>[6x]MSTLNKHISIPKDMSSKDDLDFHFLREEGIRYIKELGSNFWTDYNTHDPGITMLEVLCYAISDLGNRINIPIEDLIANEEGGVKGQFYKVQEILPSAPTSELDLRKLFIDIEGIKNCWIKRERVTVFADLKNQKLSYEKTIWEDLKENQKAQFDLKGLYRILVETEDADKVLSESLEKAVFTKFHANRNLCEDLIKVEKVATEPISVCANVEVAPEADEELIHAQILIAIEDYLAPSPRHYSLKQMVDKGYTMDEIFEGPFLENGFIDTVELKASELRKEVRLSDIINIIMSIDGVKIVKEITLGNCDENDGIENNQWVICIPENKKPKLCKKTTINYFKGILPINLNPVRVDNHKSKILASRLENDLKAKDDLEPAIPQGTFADWGEYSSIQHEFPETYGISDIGLPPKLGVKRAVLARQLKGYLLFFDQILASYFEHLSKIKSLLSLDQGPSFTYFTQAIKDIKDVEELFKDPTLLENDEELTKSLIGKLDDTIERRNQLMDHLIARFAENFSSYAFLMKFLYGESTDEIVLQDKQSFLREYKEISRERGEGFNFYEQSNDNLWDTLNVSGAQKRISKLVGVKDYSRRNLSDTAVEIYRYEHVDGNWVYRWRIRDENGKVLLSATTSYPTYNSAGNEMYFAILKILETPLSDLEKLLEVNFRNENEAGSFHFHKAATSNKFSFDIINPVIDSESSSDFIVAKQYTYYPDRTQAVLGAISLLNFIKYTFTEEGIYLVEHILLRPSPLDPEYLAMQTDAGKEYIEGNFLPFCSDDYENCKMIDPYSFRVSIVLPGFTYRFANKDFRDYLENLIREELPAHIVAKICWIGYRKGEEPELFQEDVENPETPIFKENQLEIFEKAYKNYLFELTDIHKRKGFIASMNKYNQVLNEMTSSLTGLHTIYPTGRLYDCEDEEEELDGKLILGKTNLGTL;>MSENCNHIVTTLKRDGTGRRDLLDPKLAPESVQLQDFELSDWLIFALNFARKIHFFPSDLANEPLGDWR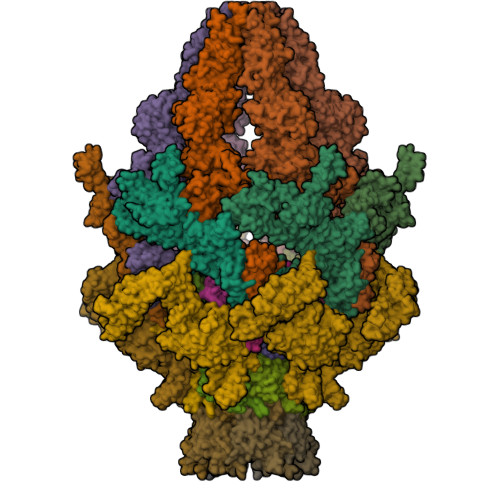NFFSTIVSDKTLISDIENLDDFEKLRGNIEEFLAAYDQSGKLTPHLTLFVSFLKLLETSKKRFNQLTKRHLDFYYQEILHLEKQALSPDHVFLIFELAKNVSQEKLDEGTEVDGGKDDTGKKNTYLTSFETVLNKTKVGQLKSLYNEISVEKEEIKELNTPISTGTFVMAPMANSFDGLGEDFPKGSEKWWPFGYTKICNASTVLPALPKARLGCSISSKLLKLSEGTRDIILEFTFNKPILPNGEDYTALNKAMSIELTGEKGWIAGLPMTLKSDSGINSGSKKMKLSLTLDSEQPAVVPYQTELHEGSYEVDEPLLRVLFKTNEKEGYNLYRLFNENVLTDLKITVEVSDITSVQLENDLGVLNPQKPFFPFGPRPIKGSSFIVKYPEAMEKPVTAISYQMDYLNLPENLVNHYSAYTIGDDEPLVSDMDYFSVKSFPKSSNDSDQLFSEKSGGGYESDFEFQIENGVWESGLKKELKISLERSFLHEKYAHYFTLVAISKDTDPTIELLPNEPYAPLAENLVLGYTAISSIDFSSSSSENQVSLIHEMPFGFQQVFTPGDTDNSLYLVPDYCHGGELYIGLENGKNLQQVTLLLQFLEGSENPDITDIFTGNQKIKWQYLSQNQWQDFQSGEIIQNQTPRFLKSGIFQFSIPKQANLDNTVLPPGYHWIKASMVKPFDVVSQLINIHAQAVEAVFEDQGSSGNHLEKGLPAETISKLQERLSWIKSIQQPYPSTKGKAQESDEDYYRRVSERLRHKKRAITLWDYEHLILQKFPKVYKVKCLNHTCSSSFQSPGNATLILVPDTVQQSVFDIYQPRVSQGTLNDVAAFVNELNSFHVQAKVINPNYEEVKVDVKVKFREGLDVSFYLTKVKEDIKKFLSPWAYDQESSVEFGVTLHRSQMIHYLEQLTYVDYITDLRLLKRQAGSSPCNPIFIETTEKEYIQPSNPKSILVSAKEHLVTPITQNCSSISLNNEEECQH[6x];>MSEGKLEKLRIVAYKDSKFSDEVENGEFITLLNPEKYKFQYRVEQNEDQASGTSSAPIRFNKILPQTLEFDFLFDRTGVIAGYEVTEDGIINDIDHFKKVVYDYNGEKHKPNYLMITWGSLLFKGYLKEMDIEYKLFRPDGTPIRAMATTKIGEFVEEELRTAQENNQSPDMSHYRTVKEGDTLPLMTYRIYGDSKYYLEVAKANGLTNFRRLKTGTELIFPPLQKQK[6x];>[6x]MMEKSKDFLGTGWGFPPEFETSIGQVKTTSGVEDIQKSLEILFSTKIGERIMQPTYGCNLDELLFSPINRTLKTYVIELIKNAILYHEPRIDPEKIDITQGNEIEGELLIHLQYIVRATNSRKNMVYPFYLEEGTNI;>[6x]MATYYPPSSFHFLVEFTGIDAKNNDHEFQSVSGLSVDIDTEEFAEGGENRFKHKFPVKTKYPNLVLKRGVLVDSKVISWCRDAIEDFEFKPIDLTVKLLNEEHQPLMTWNVVHAYPVKWSVEDFNAQESKMAIESVELSYNYFKTIV;>MATYKTPGVYIEEITKFPPSVAQVETAIPAFIGYTQFARTKPSVDSDDLILKPKRISSLLDFTTYYGGAQNEQGITVKLTDTLIEGAENRTINVPEPTFKSPYLMFYSLQMYFANGGGPCYIVSTGVYDDWSDSETPPTINFSDLESGLAVIRKEDEPTLLLFPDATNLPTDDEFYSLYNSALMQCNDLQDRFTILDTYSDQTYNDGVEDLDPIPALRNGINLTKDYLKYGAAYYPFVQTILNYQYSADEIVIQHLSYNPNAIATALDNLNAVNGPTFIDAILDDLRDLSLPDISGEISDAVGFMYDDVDGFDIDGTFTTNSVKVANFASLVESVLSTLNELIDAKEEINKDVNSAIASSEEDNAIKTAISDALDVFNEDFEGADKIESVAKNLSDLLIKIKQADTNTKVENVLSINALNFSAEFEKLLTYDVNTGLTASVTLDLFANIGTRLDDIIAAVSAAEPIDVNNGKLNGRLLSDIEPLDNATYNTILLEINSHKVTLPPSSSMAGAYARVDNDRGVWKSPANIGLNYVSKPSVTVSHEEQESMNVHGTGKSVNAIRSFVGKGTLVWGARTLAGNDNEWRYISVRRFFNMAEESIKKATEQFVFEPNDGNTWVRVRAMIENFLILQWRAGALAGAKPEHAFYVKVGLGQTMTAQDILEGNMNVEIGLAVVRPAEFIILKFSHKMQES[6x];>MSYPLSKFHFSVEWGGTKIGFTEVSGLDLETEIIEYRHGASPEYSKIKMPGMQKFSNITLKRGTFKSDNEYFQWYNTINLNKVERRDLTISLLNEEHEPVVTWKVKNAWPLKVQSTDLKGDGNEVAIESMELAHEGLVIQNE[6x]>MHRYSRTGKHRWTVRALAVLFTALLGLTQWTAPASAHGSVINPATRNYGCWLRWGHDHLNPNMQYEDPMCWQAWQDNPNAMWNWNGLYRDWVGGNHRAALPDGQLCSGGLTEGGRYRSMDAVGPWKTTDVNNTFTIHLYDQASHGADYFLVYVTKQGFDPTTQPLTWDSLELVHQTGSYPPAQNIQFTVHAPNRSGRHVVFTIWKASHMDQTYYLCSDVNFV[2x]

Lytic polysaccharide monooxygenases (LPMOs) are auxiliary activity enzymes that also attack cellulose, as well as other polysaccharides, using an oxidative mechanism. LPMOs are compact globular enzymes that lack a substrate binding cleft or tunnel, and instead have a copper atom containing active site located near a planar binding surface. Thermobifida fusca, a model cellulolytic bacterium, secretes two LPMOs, the type I (TfAA10B) and type III (TfAA10A). The first LPMO structure to be solved was the chitinolytic LPMO SmCBP21 and more recently several bacterial LPMOs acting on cellulose have been investigated. These structures share a common immunoglobulin-like β-sandwich core fold, a flat binding surface, and a conserved N-terminal histidine.

The structure of TfAA10A was refined to a resolution of 2.0 Å with R and Rfree of 0.167 and 0.233, respectively. There are two molecules in the asymmetric unit with two copper atoms and multiple iodides. It has an Ig-like β-sandwich fold with a copper ion bound on the active site. A histidine brace, a conserved feature of LPMOs coordination with copper, facilitated by the N-terminal histidine 37 can be clearly observed in TfAA10A. An interesting feature of TfAA10A is the axial position of the copper coordination sphere, which is tyrosine. In most AA10 LPMOs and in TfAA10B, a phenylalanine occupies this position. The copper atom at the active site of chain A is 50% occupied and the one with chain B has occupancy of 31%. The active site of chain A has type I copper coordination in agreement with previous studies while the more distorted active site of chain B includes some features similar to type 2 with an equatorial water (wat550) in contact with the copper. Clearly, both active sites have been photo-reduced by X-ray radiation during data collection supporting the assumption that copper(II) is the catalytically competent state. Closer comparison between the Streptomyces coelicolor lytic polysaccharide monooxygenase and TfAA10A reveals almost identical backbone and His144, Tyr213, Trp82 and Asn83 at the same locations and conformations.> MARAAFLFKTVGFGGLQNVPINDELSSHLLRAGNSPWQLTQFLDWISLGRGLATSALVPTAGSRYYQMSCLLSGTLQIPFRPNHRWGDIRFLRLVWSAPTLDGLVVAPPQVLAQPALQAQADRVYDCDDYPFLARDPRFKHRVYQQLSAVTLLNLTGFGPISYVRVDEDMWSGDVNQLLMNYFGHTFAEIAYTLCQASANRPWEHDGTYARMTQIILSLFWLSYVGVIHQQNTYRTFYFQCNRRGDAAEVWILSCSLNHSAQIRPGNRSLFVMPTSPDWNMDVNLILSSTLTGCLCSGSQLPLIDNNSVPAVSRNIHGWTGRAGNQLHGFQVRRMVTEFCDRLRRDGVMTQAQQNQIEALADQTQQFKRDKLEAWAREDDQYNQANPNSTMFRTKPF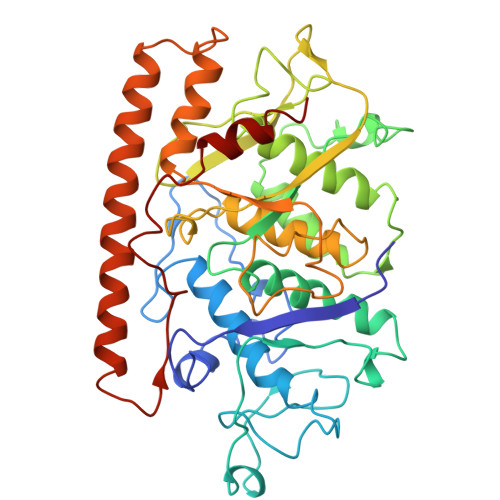TNAQWGRGNTGATSAAIAALI> GPLGSEEIKNIDAKIRKWSSGKSGNIRSLLSTLQYILWSGSGWKPVPLMDMIEGNAVRKSYQ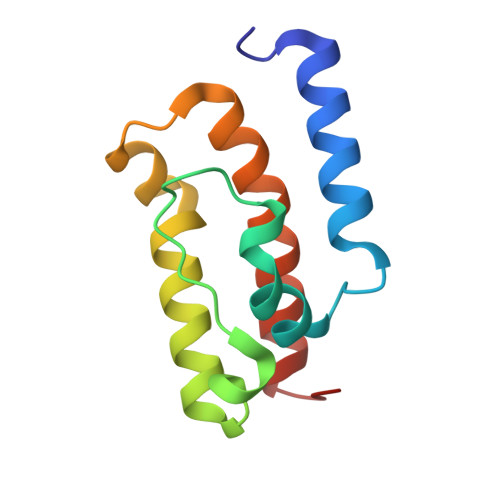RALLILHPDKLQQKGASANQKYMAEKVFELLQEAWDHFNTLGPV> CTPSR;> LAHSKMVPIPAGVFTMGTDDPQIKQDGEAPARRVTIDAFYMDAYEVSNTEFEKFVNSTGYLTEAEKFGDSFVFEGMLSEQVKTNIQQAVAAAPWWLPVKGANWRHPEGPDSTILHRPDHPVLHVSWNDAVAYCTWAGKRLPTEAEW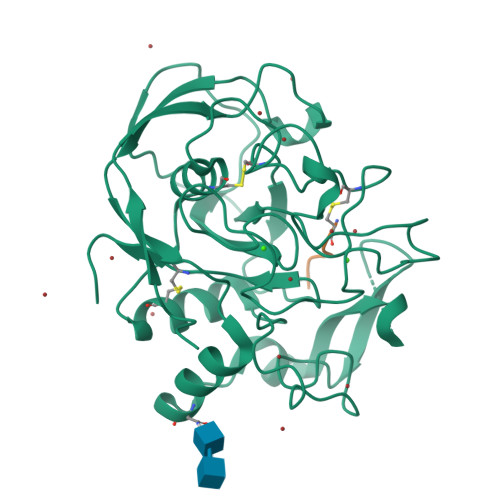EYSCRGGLHNRLFPWGNKLQPKGQHYANIWQGEFPVTNTGEDGFQGTAPVDAFPPNGYGLYNIVGNAWEWTSDWWTVHHSVEETLNPKGPPSGKDRVKKGGSYMSHRSYCYRYRCAARSQNTPDSSASNLGFRCAADRLP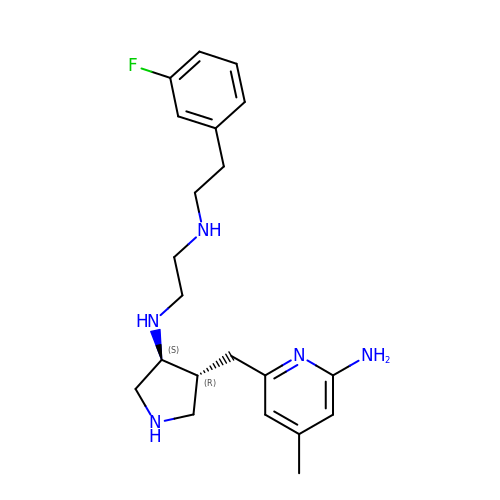N-{(3S,4R)-4-[(6-amino-4-methylpyridin-2-yl)methyl]pyrrolidin-3-yl}-N'-[2-(3-fluorophenyl)ethyl]ethane-1,2-diamine | C21 H30 F N5 | PUOKPLCASUFBAN-YLJYHZDGSA-N> GGILDPANGNSHAYFNIDEVRSKNVLKQITQLINEVTNITETFPLKPGQTTEGLVATLDAAVANFLQTGSFAISKCPIANSDPRAIDLLHEALGAVQDTGQVMIQTGRDF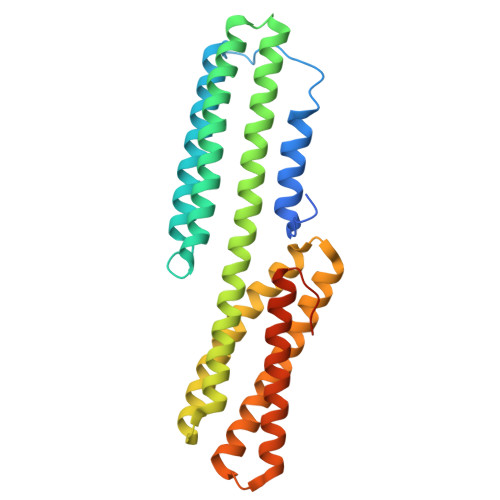VRDSTSTNKRAIATNSGRNLLTAVAKFLILADSIDVKVIVDKVDEVRETAHQMIEADTKIKVDDLYNLLISQIEELDITVRRRAIDLVKPNQRDDLLAARSALRQTAPLLYTSTRTFVRHPEHEEARRNRDYTADEMHSALNALESVLNGQQPKVTFSEYGRIGDLINE> MSLSNKLTLDKLDVKGKRVVMRVDFNVPMKNNQITNNQRIKAAVPSIKFCLDNGAKSVVLMSHLGRPDGVPMPDKYSLEPVAVELKSLLGKDVLFLKDCVGPEVEKACANPAAGSVILLENLRFHVEEEGKGKDASGNKVKAEPAKIEAFRASLSKLGDVYVNDAFGTAHRAHSSMVGVNLPQKAGGFLMKKELNYFAKALESPERPFLAI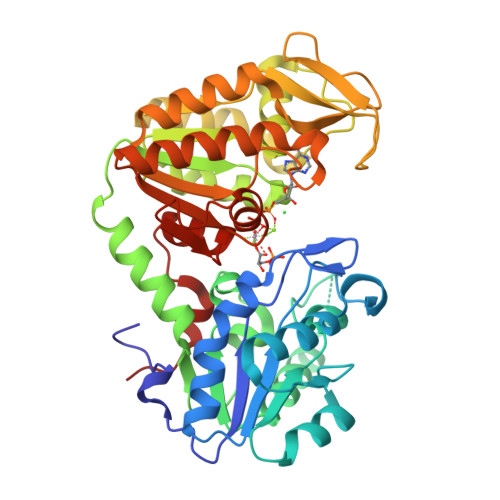LGGAKVADAIQLINNMLDKVNEMIIGGGMAFTFLKVLNNMEIGTSLFDEEGAKIVKDLMSKAEKNGVKITLPVDFVTADKFDENAKTGQATVASGIPAGWMGLDCGPESSKKYAEAVTRAKQIVWNGPVGVFEWEAFARGTKALMDEVVKATSRGCITIIGGGDTATCCAKWNTEDKVSHVSTGGGASLELLEGKVLPGVDALSNI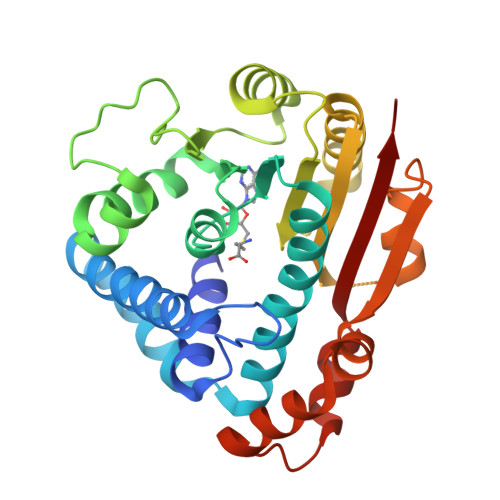> MERIIQQTDYDALSCKLAAISVGYLPSSGLQRLSVDLSKKYTEWHRSYLITLKKFSRRAFGKVDKAMRSSFPVMNYGTYLRTVGIDAAILEFLVANEKVQVVNLGCGSDLRMLPLLQMFPHLAYVDIDYNESVELKNSILRESEILRISLGLSKEDTAKSPFLIDQGRYKLAACDLNDITETTRLLDVCTKREIPTIVISECLLCYMHNNESQLLINTIMSKFSHGLWISYDPIGGSQPNDRFGAIMQSNLKESRNLEMPTLMTYNSKEKYASRWSAAPNVIVNDMWEIFNAQIPESERKRLRSLQFLDELEELKVMQTHYILMKAQWHHHHHH For example, there are significant differences in the annotations and even in the sequences of particular proteins. This is especially true of 30-kDa lipoproteins (30-kDa LPs), the most abundant group of proteins found in the hemolymph of the silkworm fifth instar larvae. The 30-kDa LPs are involved in many physiological processes in the silkworm body. They transport lipids in the hemolymph, tryptophan metabolites and pigments in diapause silkworm eggs, are involved in an immune response pathway in an antifungal defense system, serve as the source of nutrients during pupation and adult development, and are the second major yolk protein component. Bmlp6, as a 30-kDa LP member, has a fold characteristic of this protein family, classified as Lipoprotein_11 family (Pfam: PF03260). Thus, Bmlp6 is composed of two domains, the N-terminal VHS domain (Pfam: PF00790) and the C-terminal β-trefoil domain (Pfam: PF14200).

Here we present the crystal structure of Bombyx mori lipoprotein 6 (Bmlp6). Bmlp6 crystallized in space group P21. The crystal structure of 1.8 Å resolution shows five copies of a two-domain molecule with a typical 30-kDa LP fold. The N-terminal domain (NTD) of Bmlp6 (residues 1-91) consists of six helices forming a right-handed superhelix and packed in a globular form. The C-terminal domain (CTD) of Bmlp6 (residues 92–245) is folded as a ricin-type β-trefoil lectin-like domain. The interactions between the monomers in the crystal lattice are weak with no indication of possible quaternary structure, as established by the PISA server. Specifically, molecules of MES, isopropanol and fragments of PEG were mainly located at the protein surface. There are only two potential cavities in Bmlp6, denoted Po.1 and Po.2, in contrast to Bmlp3 and Bmlp7, where three cavities (No. 1–3) are present. The structure demonstrates that Bmlp6 differs from Bmlp3 and Bmlp7 in the conformation of loops, the electrostatic surface potential, and potential binding cavities.

>[5x]GVVELSADTSNQDLEEKLYNSILTGDYDSAVRQSLEYESQGKGSIIQNVVNNLIIDKRRNTMEYCYKLWVGNGQEIVRKYFPLNFRLIMAGNYVKIIYRNYNLALKLGSTTNPSNERIAYGDGVDKHTELVSWKFITLWENNRVYFKIHNTKYNQYLKMSTTTCNCNSRDRVVYGGNSADSTREQWFFQPAKYENDVLFFIYNRQFNDALELGTIVNASGDRKAVGHDGEVAGLPDIYSWFITPF>MT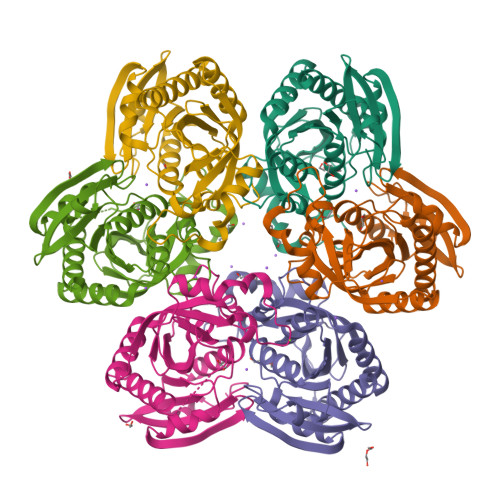KTVFHLGVTEADLNGATLAIIPGDPARVQKIAELMDNPVFLASHREYTVYRAELDGQSVVVCSTGIGGPSTSIAVEELAQLGVRTFLRVGTTGAIQPHVNVGDMIVTTGSVRLDGASLHFAPMEFPAVPDFDVATAMKAAAQESGATVHMGVTASSDTFYPGQERYDTFTGRVVRRFQGSMKEWQDMGVLNFEMESATLLTMCASSGLKAGCVAGVIINRTQKEIPDHATLKETEARSIKVVVEAARKMLK[6x]> MHHHHHHGENLYFQGSGVEVIFYLSDREPLRLGSGEYTAEELCIRAAQACRISPLCHNLFALYDENTKLWYAPNRTITVDDKMSLRLHYRMRFYFTNWHGTNDNEQSVWRHSPKKQKNGYEKKKIPDATPLLDASSLEYLFAQGQYDLVKCLAPIRDPKTEQDGHDIENECLGMAVLAISHYAMMKKMQLPELPKDISYKRYIPETLNKSIRQRNLLTRMRINNVFKDFLKEFNNKTICDSSVSTHDLKVKYLATLETLTKHYGAEIFETSMLLISSENEMNWFHSNDGGNVLYYEVMVTGNLGIQWRHKPNVVSVEKEKNKLKRKKLENKDKKDEEKNKIREEWNNFSFFPEITHIVIKESVVSINKQDNKKMELKLSSHEEALSFVSLVDGYFRLTADAHHYLCTDVAPPLIVHNIQNGCHGPICTEYAINK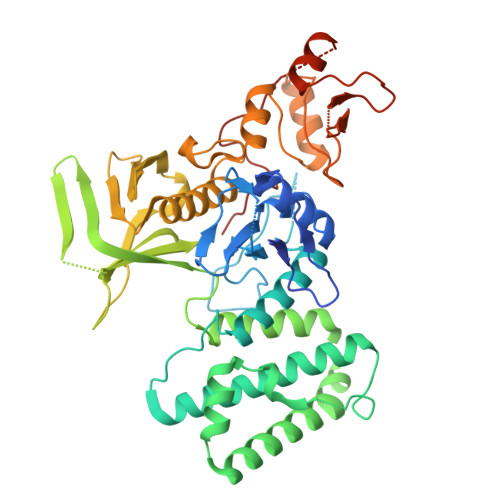LRQEGSEEGMYVLRWSCTDFDNILMTVTCFEKSEQVQGAQKQFKNFQIEVQKGRYSLHGSDRSFPSLGDLMSHLKKQILRTDNISFMLKRCCQPKPREISNLLVATKGNS> MAESKPTPQSTFTGPIVVDPITRIEGHLRIMVEVENGKVKDAWSSSQLFRGLEIILKGRDPRDAQHFTQRACGVCTYVHALASSRCV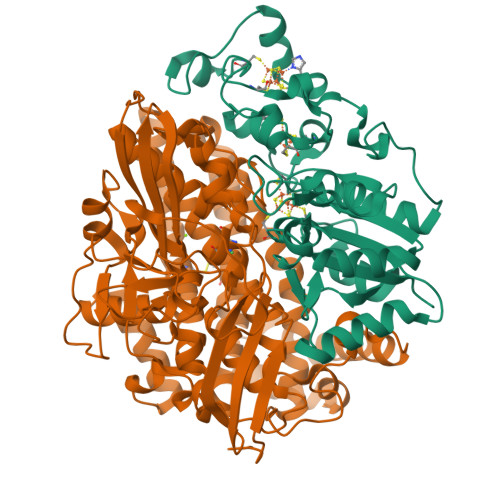DDAVKVSIPANARMMRNLVMASQYLHDHLVHFYHLHALDWVDVTAALKADPNKAAKLAASIDTARTGNSEKALKAVQDKLKAFVESGQLGIFTNAYFLGGHKAYYLPPEVNLIATAHYLEALHMQVKAASAMAILGGKNPHTQFTVVGGCSNYQGLTKDPLANYLALSKEVCQFVNECYIPDLLAVAGFYKDWGGIGGTSNYLAFGEFATDDSSPEKHLATSQFPSGVITGRDLGKVDNVDLGAIYEDVKYSWYAPGGDGKHPYDGVTDPKYTKLDDKDHYSWMKAPRYKGKAMEVGPLARTFIAYAKGQPDFKKVVDMVLGKLSVPATALHSTLGRTAARGIETAIVCANMEKWIKEMADSGAKDNTLCAKWEMPEESKGVGLADAPRGSLSHWIRIKGKKIDNFQLVVPSTWNLGPRGPQGDKSPVEEALIGTPIADPKRPVEILRTVHAFDPCIACGVHVIEPETNEILKFKVC;> LTAKHRPSVVWLHNAECTGCTEAAIRTIKPYIDALILDTISLDYQETIMAAAGETSEAALHEALEGKDGYYLVVEGGLPTIDGGQWGMVAGHPMIETCKKAAAKAKGIICIGTCSPYGGVQKAKPNPSQAKGVSEALGVKTINIPGCPPNPINFVGAVVHVLTKGIPDLDENGRPKLFYGELVHDNCPRLPHFEASEFAPSFDSEEAKKGFCLYELGCKGPVTYNNCPKVLFNQVNWPVQAGHPCLGCSEPDFWDTMTPFYEQG> GRKKIQISRILDQRNRQVTFTKRKFGLMKKAYELSVLCDCEIALIIFNSANRLFQYASTDMDRVLLKYT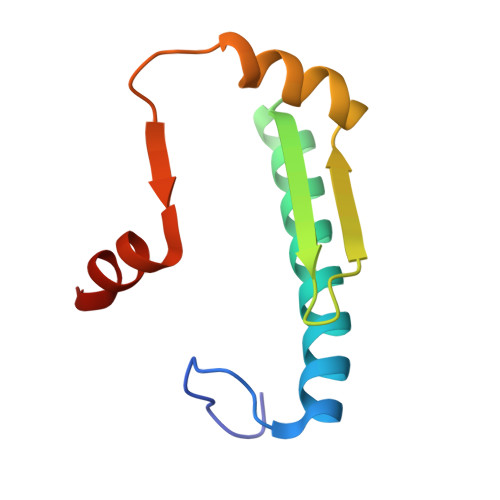EYSEPHESRTNTDILETLKRR>MFDKDNYALGKMKNTLNTKESKFSLKSTDDLNKCIDHISVLIKDAYLLYTNESFATSTFISITIIEEVGKTHIGMFISENKDIKRGKDPLRNHKSKHAFGSLPTIKMGGRLNKAIGDEMIDKIVEDAETGELISIRESSLYADIIDDILEVPSEKISKEQSRALLLYAIECFDDSLVGYTHHSFEVSETTDELFEKLAN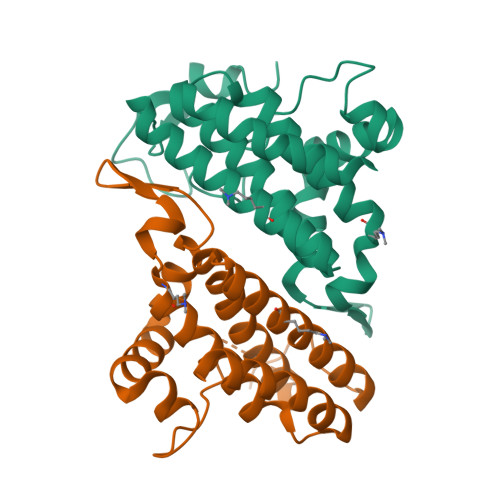NKHHHHHH[4x]>[2x]TKLNGMVLL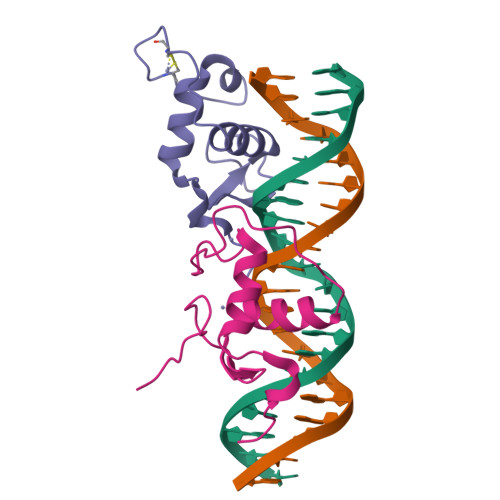CKVCGDVASGFHYGVLACEGCKGFFRRSIQQNIQYKRCLKNENCSIVRINRNRCQQCRFKKCLSVGMSRDAVRFGRIPKREKQRM>[2x]GQKLSAYVVDWDLPKSIAWDKLDHIVYA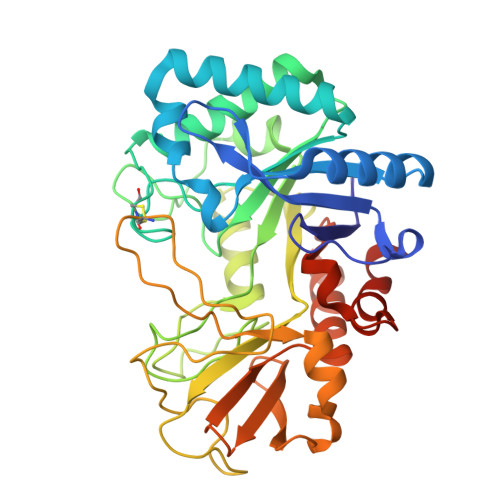FAEPTKDGELSGFTDSQLKSVVQEAHSRGKSISLSVGGWTGSLYFSDLLKSSSSFDNFVSNLVDVVKEYDLDGLNLDWEYPNSPNGVACNSKDENDTANYLKLFKALREKLGSKTILTTAVPTAPFNDENQQPSTKLDDNWASTVDAFYIMAYDVNGIRDKNAGANAPLYYSPKVTGVEPTSGNDAVKAWIAAGIPAEQLVLGVPFYGRVSKTLEPITASTGLYVPISQSSQIKGDSTDEKAADPCPNAVATYSGQYIWRTIAQEGIARNSSGWVTYWDDISKTPYAYSFSGSKVLSFDDAASLQDKVDYAKKQGLGGVMLWSLEMDDDENTLLNALQDIRKLGHHHHHH>MANMKNSNDRIILFRKAGEKVDATKMLFLTEYGLSHEADTDTEDTMDGSYNTGGSVESTMSGTAKMFYGDDFADEIEDAVVDRVLYEAWEVESRIPGKNGDSAKFKAKYFQGFHNKFELKAEANGIDEYEYEYGVNGRFQRGFATLPEAVTKKLKATGYRFHDTTKEDALTSEDLTAIPQPKVDSSTVTPGEV[12x];>[6x]MDIELTKKDGTVIKLSEYGFIVNDIVIDSMQINTKYQDKENMNGRILMGSNYISRDIVVPCFCKVKNRSDIAYMRDMLYSLTTDIEPMYLREIRRKEELNYRFTQPTSDDYVKLDKNNFPDYEYSRHDQQIYVNGKQYKVIFNGVINPKQKGNKVSFELKFETTELPYGESIGTSLELEENKKVGLWSFDFNIDWHAGGDKRKYTFENLSKGTVYYHGSAPNDQFNMYKKITIILGEDTESFVWNLTHAEIMKIEGIKLKAGDRIVYDSFRVYKNGVEISTETNISQPKFKYGANKFEFNQTVQKVQFDLKFYYK;>[3x]MTITIKPPKGNGAPVPVETTLVKKVNADGVLTFDILENKYTYEVINAIGKRWIVSHVEGENDKKEYVITVIDRKSEGDRQLVECTAREIPIDKLMIDRIYVNVTGSFTVERYFNIVFQGTGMLFEVEGKVKSSKFENGGEGDTRLEMFKKGLEHFGLEYKITYDKKKDRYKFVLTPFANQKASYFISDEVNANAIKLEEDASDFATFIRGYGNYSGEETFEHAGLVMEARSALAEIYGDIHAEPFKDGKVTDQETMDKELQSRLKKSLKQSLSLDFLVLRESYPEADPQPGDIVQIKSTKLGLNDLVRIVQVKTIRGINNVIVKQDVTLGEFNREQRYMKKVNTAANYVSGLNDVNLSNPSKAAENLKSKVASIAKSTLDLMSRTDLIEDKQQKVSSKTVTTSDGTIVHDFIDKSNIKDVKTIGTIGDSVARGSHAKTNFTEMLGKKLKAKTTNLARGGATMATVPIGKEAVENSIYRQAEQIRGDLIILQGTDDDWLHGYWAGVPIGTDKTDTKTFYGAFCSAIEVIRKNNPASKILVMTATRQCPMSGTMIRRKDTDKNKLGLTLEDYVNAQILACSELDVPVYDAYHTDYFKPYNPAFRKSSMPDGLHPNERGHEVIMYELIKNYYQFYG;>[3x]MTEYKIKATIEASVAKFKRQIDSAVKSVQRFKRVADQTKDVELNANDKKLQKTIKVAKKSLDAFSNKNVKAKLDASIQDLQQKILESNFELDKLNSKEASPEVKLQKQKLTKDIAEAENKLSELEKKRVNIDVNADNSKFNRVLKVSKASLEALNRSKAKAILDVDNSVANSKIKRTKEELKSIPNKTRSRLDVDTRLSIPTIYAFKKSLDALPNKKTTKVDVDTNGLKKVYAYIIKANDNFQRQMGNLANMFRVFGTVGSNMVGGLLTSSFSILIPVIASVVPVVFALLNAIKVLTGGVLALGGAVAIAGAGFVAFGAMAISAIKMLNDGTLQASSATNEYKKALDGVKSAWTDIIKQNQSAIFTTLANGLNTVKTAMQSLQPFFSGISRGMEEASQSVLKWAENSSVASRFFNMMNTTGVSVFNKLLSAAGGFGDGLVNVFTQLAPLFQWSADWLDRLGQSFSNWANSAAGENSITRFIEYTKTNLPIIGNIFKNVFAGINNLMNAFSGSSTGIFQSLEQMTAKFREWSEQVGQSQGFKDFVSYIQTNGPLIMQLIGNIARGLVAFATAMAPIASAVLRVAVAITGWIANLFEAHPATAQLVGVIITLVGAFRFLIAPILAVMDFLGPLAARLVALVTKFGWAKTGTLVLSKAMTSLKGPIKLVTAIFQLLFGKIGLIRNAITGLVTVFGILGGPITIVIGVIAALIAIFVLLWNKNEGFRNFIINAWNAIKTFMVNVWNVLKAVASVVWNAILTAITTAVSNVYNFIMIVWNQIVAYLQGLWNGIIAIATTVWNLLVTIITTVFTTIMTIVMTIWTAIWTFLSTIWNTIITIATTIWNLLVTVITTVFTTIMTIAMTIWNAIWTFLQTLWNTIVTVATKVWNAITTAISTALQAAWSFISNIWNTIWSFLSGILTTIWNKVVSIFTQVVSTISDKMSQAWNFIVTKGMQWVSTITSTLINFVNRVIQGFVNVVNKVSQGMTNAVNKIKSFIGDFVSAGADMIRGLIRGIGQMAGQLVDAAKNVAKKALDAAKSALGIHSPSREFMDVGMYSMLGFVKGIDNHSSKVIRNVSNVADKVVDAFQPTLNAPDISSITGNLSNLGGNINAQVQHTHSIETSPNMKTVKVEFDVNNDALTSIVNGRNAKRNSEYYL;>[18x]MDNKLITDLSRVFDYRYVDENEYNFKLISDMLTDFNFSLEYHRNKEVFAHNGEQIKYEHLNVTSSVSDFLTYLNGRFSNMVLGHNGDGINEVKDARVDNTGYDHKTLQDRLYHDYSTLDAFTKKVEKAVDENYKEYRATEYRFEPKEQEPEFITDLSPYTNAVMQSFWVDPRTKIIYMTQARPGNHYMLSRLKPNGQFIDRLLVKNGGHGTHNAYRYIGNELWIYSAVLDANENNKFVRFQYRTGEITYGNEMQDVMPNIFNDRYTSAIYNPIENLMIFRREYKASERQLKNSLNFVEVRSADDIDKGIDKVLYQMDIPMEYTSDTQPMQGITYDAGILYWYTGDSKPANPNYLQGFDIKTKELLFKRRIDIGGVNNNFKGDFQEAEGLDMYYDLETGRKALLIGVTIGPGNNRHHSIYSIGQRGVNQFLKNIAPQVSMTDSGGRVKPLPIQNPAYLSDITEVGHYYIYTQDTQNALDFPLPKAFRDAGWFFDVLPGHYNGALRQVLTRNSTGRNMLKFERVIDIFNKKNNGAWNFCPQNAGYWEHIPKSITKLSDLKIVGLDFYITTEESNRFTDFPKDFKGIAGWILEVKSNTPGNTTQVLRRNNFPSAHQFLVRNFGTGGVGKWSLFEGKVVE;>MVVDNFSKDDNLIELQTTSQYNPVIDTNISFYESDRGTGVLNFAVTKNNRPLSISSEHVKTFIVLKTDDYNVDRGAYISDELTIVDAINGRLQYVIPNEFLKHSGKVHAQAFFTQNGSDNVVVERQFSFNIENDLVSGFDGITKLVYIKSIQDTIEAVGKDFNQLKQNMADTQTLIAKVNDSATKGIQQIEIKQNEAIQAITATQTSATQAVTAEFDKIVEKEQAIFERVNEVEQQINGADLVKGNSTTNWQKSKLTDDYGKAIESYEQSIDSVLSAVNTSRIIHITSATDAPSFKDIGTVDTPKEDGVDDGSDIPVAPNTLGKSGVLVVYVVDDSTARATWYPDDSNDEYTKYKISGTWYPFYKKNDGDLTKQFVEETSNNALNQAKQYVDDKFGTTSWQQHKMTEANGQSIQVNLNNAQGDLGYLTAGNYYATRVPDLPGSVESYEGYLSVFVKDDTNKLFNFTPYNSKKIYTRSITNGRLEQQWTVPNEHKSTVLFDGGANGVGTTINLTEPYTNYSILLVSGTYPGGVIEGFGLTALPNAIQLSKANVVDSDGNGGGIYECLLSKTSSTTLRIDNDVYFDLGKTSGSGANANKVTITKIMGWK[18x];>[12x]MYKIKDVETRIKNDGVDLGDIGCRFYTEDENTASIRIGINDKQGRIDLKAHGLTPRLHLFMEDGSIFKNEPLI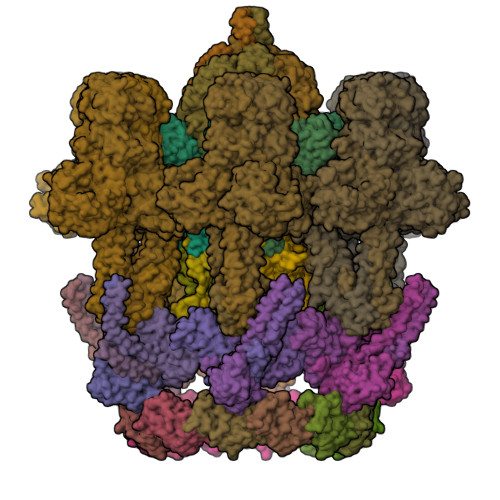IDDVVKGFITYKIPKKVIKHAGYVRCKLFLEKEEEKIHVANFSFNIVDSGIESAVAKEIDVKLVDDAITRILKDNATDLLSKDFKEKIDKDVISYIEKNESRFKGAKGDKGEPGQPGAKGEAGKKGEQGAPGKNGTVVSINPDTKMWQIDGKDTDIKAEPELLDKINIANVEGLEDKLQEVEKIKDTTLNDSKTYTDTKIAELVDSAPESMNTLRELAEAIQNNSISESVLQQIGSKVSTEDFEEFKQTLNDLYAPKNHNHDERYVLSSQAFTKQQADSLYQLKSASQPTVKIWTGTENEYNYIYQKDPNTLYLIKG>GSHMNTEVSSEIYQWVRDELKRAGISQAVFARVAFNRTQGLLSEILRKEE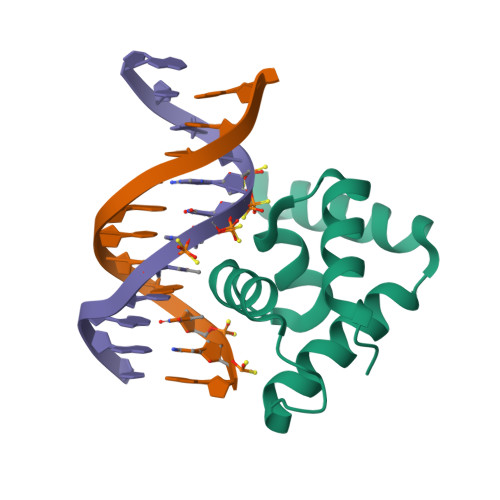DPKTASQSLLVNLRAMQNFLQLPEAERDRIYQDERERSLRKRK[2x]> GIEASLLTDPKDVSGRTVDYIIAGGGLVGLTTAARLTENPNISVLVIESGSYESDRGPIIEDLNAYGDIFGSSVDHAYETVELATNNQTALVRSGNGLGGSTLVNGGTWTRPHKAQVDSWETVFGNEGWNWDNVAAYSLQAERARAPNAK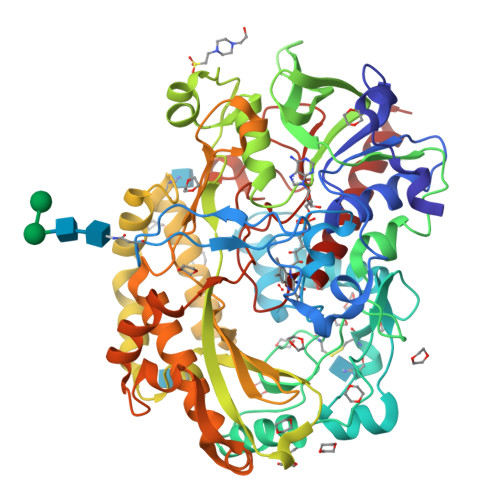QIAAGHYFNTSCHGVNGTVHAGPRDTGDDYSPIVKALMSAVEDRGVPTKKDFGCGDPHGVSMFPNTLHEDQVRSDAAREWLLPNYQRPNLQVLTGQYVGKVLLSQNGTTPRAVGVEFGTHKGNTHNVYAKHEVLLAAGSAVSPTILEYSGIGMKSILEPLGIDTVVDLPVGLNLQDQTTATVRSRITSAGAGQGQAAWFATFNETFGDYSEKAHELLNTKLEQWAEEAVARGGFHNTTALLIQYENYRDWIVNHNVAYSELFLDTAGVASFDVWDLLPFTRGYVHILDKDPYLHHFAYDPQYFLNELDLLGQAAATQLARNISNSGAMQTYFAGETIPGDNLAYDADLSAWTEYIPYHFRPNYHGVGTCSMMPKEMGGVVDNAAKVYGVQGLRVIDGSIPPTQVSSHVMTVFYAMALKISDAILEDYASMQ>MVIKFGYKASAEQFGPRELVELGVLAEAHGMDSATVSDHFQPWRHEGGHAPFSLAWMTAVGERTSRLQLGTSVMTPTFRYNPAVVAQAFATMGCLYPGRIMLGVGTGEALNEIATGFAGEWPEFKERFARLREAVALMRELWLGDRVDFEGNYYKTVGASIYDVPEGGIPVYIAAGGPVVARYAGRSGDGFICTSGKGMELYTEKLMPAVAEGAEKADRDVAEIDKMIEIKISYDTDPELALENTRFWAPLSLTPEQKHSIDDPIEMERAADALPIEQVAKRWIVASDPDEAVAQIRPYLDAGLNHLVFHAPGHDQKRFLELFQRDLAPRLRGLA[2x]

In mycobacteria and other actinomycetes, glucose-6-phosphate dehydrogenases (FGDs) seem to be the main producer of F420H2, by catalyzing the reaction F420 + glucose-6-phosphate → F420H2 + 6-phosphogluconolactone. Since the identification of the first FGD two decades ago in Daniels’ lab, only two FGDs from actinomycetes, namely M. smegmatis and Mtb, have been characterized in detail. These two FGDs share 37% sequence similarity and belong to an F420-dependent enzyme subgroup within the luciferase-like hydride transferase family. Rh-FGD1 is strictly dependent on F420 as coenzyme. Rh-FGD1 was also found to be highly specific for G6P as electron donor.

We have focused our exploration on Rh-FGD1, the best expressed one, characterized the kinetic properties and elucidated the structure of the apo protein at high resolution. The asymmetric unit contains two enzyme monomers forming a compact dimer, which is also observed in solution as estimated by gel permeation analysis (data not shown), similarly to the mycobacterial homolog (1.0 Å rmsd difference for 610 pairs of Cα atoms). Each Rh-FGD1 monomer is comprised of residues 1–334, forming an (α/β)8 TIM-barrel, with the active site typically located at the C-terminus of the barrel, as observed in Mtb-FGD1. Only residues 254–263 in subunit A, and 250–279 in subunit B lack clear electron density and were therefore excluded from the final model. In particular, the high - quality electron density clearly indicates the presence of a well-ordered nonprolyl cis-peptide bond between Ser72–Val73 constituent of a bulge at the end of a β strand close to the presumed binding site of the F420 isoalloxazine ring. All attempts to elucidate the structure of Rh-FGD1 in its holoenzyme form, i.e., with the F420 cofactor bound, were unsuccessful. Nonetheless, the obtained overall structure is substantially identical to that of the F420-bound Mtb-FGD1 and the architecture of the active site is conserved. In Rh-FGD1, the sequence for this structural element is shorter than that of the homologous enzymes and corresponds to the disordered part (residues 254–263 in monomer A). In Rh-FGD1, out of the three residues, the position of Lys258 is unknown as it is part of the disordered region.>HHHHHHSSGLVPRGSHMLLTADTVLTGTELLRPGWLEIASDRVVAVGAGAPPAQADRNLGAATVVPGFVDTHLHGGGGGNFSAATDDETARAVALHRAHGSTTLVASLVTAGPEDLLRQVSGLARQVRAGLIDGIHLEGPWLSTLRCGAHQPVLMRDPDPGEIGRVLDAGEGTVRMVTIAPERDGALAAIAQLVNAGVVAAVGHTEATYDQTRAAIDAGATVGTHLFNAMRPIDRREPGPAVALTEDSRVTVEMIVDGVHVAPAIYRHITQTVGPERLSLITAAMAATGMSDGVYRLGPLDIDVVAGVARVAGTDTIAGSTATMEQVFRLAVAHCGLPRDDALSLAVRQACVNPARALGLPAAGLAAGARADLVVLDHDLAVTAVMRAGEWVVTPGAAHTV[2x]

NagA enzymes (EC 3.5.1.25) are widespread in nature and found in a range of eukaryotic and prokaryotic species as metal-dependent enzymes with a physiological role in catalyzing the deacetylation of GlcNAc6P to yield GlcN6P and acetate. Our X-ray crystallographic structure determination reveals that MSNagA conforms to the urease structural superfamily, with the same overall fold, domain topology, and architecture as other NagA enzymes whose structures have been determined. Domain I (residues 52–344) is a twisted (β/α)8-TIM barrel that is comprised of eight alternating β-stands and α-helices and encloses the catalytic site of the enzyme and the metal-binding site. Domain II is a small β-barrel comprising eight β-strands contributed from the N and C termini of the MSNagA protein (amino acids 1–51 and 344–382).

To investigate the interaction of the GlcNAc6P substrate with the protein, we mutated Asp-267, which has been shown to be important for catalysis in other NagA enzymes, to alanine. This resulted in significant loss of enzymatic activity and enabled co-crystallization of the MSNagA enzyme in the presence of GlcNAc6P. The structure was solved by molecular replacement using the apo-MSNagA as a model and refined at a resolution of 2.0 Å. The co-crystal structure shows clear electron density for GlcNAc6P in the substrate-binding pocket of Chain A, enabling the substrate to be modeled in the active-site pocket at the dimeric interface. However, it may be that the site is not fully occupied, and no electron density for the GlcNAc6P substrate was observed in the second active site of chain B where instead a flexible loop region from Glu-122 to Pro-136 partially occludes the active site. The GlcNAc6P substrate is situated in the cavity of the (α/β) barrel of domain I at the dimer interface, recruiting Arg-219 from the opposing monomer through an interaction with the phosphate moiety. The GlcNAc6P substrate is found in the α-configuration and is anchored in place through the formation of hydrogen bonds with the side chains of His-244 that interacts with the anomeric GlcNAc6P hydroxyl group and with Asn-212 to the phosphate group. The carbonyl group of the GlcNAc6P substrate is positioned ∼2.5 Å from the M1 metal ion, which is ideally primed to stabilize the transition state intermediate formed during catalysis. We therefore modeled a cadmium ion at this position, which is likely to arise as a result of the addition of CdCl2 in the crystallization conditions with the metal-binding site perhaps being destabilized by the D267A mutation. The M2 metal ion is similarly coordinated to Glu-122, His-188, and His-209, and it is striking that an additional interaction is formed with the carbonyl group of the GlcNAc6P substrate, replacing the water molecule in the apo-structure.> MGSSHHHHHHSSGRENLYFQGMSLEPFGARLSRAMDDRGPLCVGIDPHASLLADWGLSDDVAGLERFSRTVVEALGEHVAVFKPQSAFFERFGSRGVAVLEKTVAEARAAGALVVMDAKRGDIGSTMAAYAEAFLRKDSPLFSDALTVSPYLGYGSLRPAVELARESGAGLFVLALTSNPEGGEVQHAVRTDGRDVAATMLAH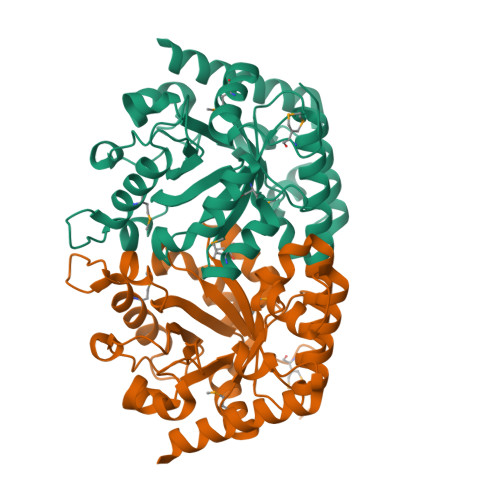LAAENAGEEPLGSFGAVVGATLGDLSSYDLDINGPLLAPGIGAQGAAPADLPGVFGAAVRNVVPNVSRGVLRHGPDVRALRTAADRFAEEIRAAVAAV>[2x]SDKP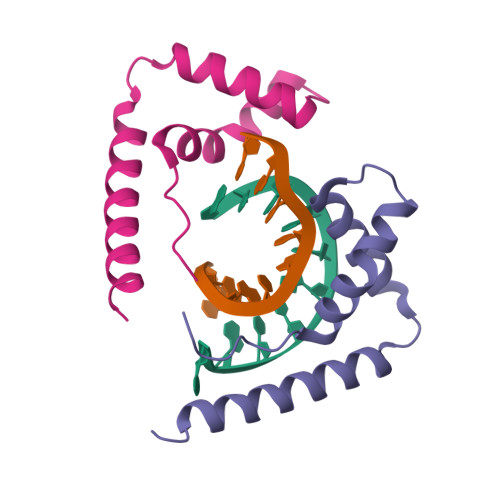KRPLSAYMLWLNSARESIKRENPGIKVTEVAKRGGELWRAMKDKSEWEAKAAKAKDDYDRAVKEFEANG> MGERPPPKRLTREAMRNYLKERGDQTVLILHAKVAQKSYGNEKRFFCPPPCVYLMGSGWKKKKEQMERDGCSEQESQPCAFIGIGNSDQEMQQLNLEGKNYCTAKTLYISDSDKRKHFMLSVKMFYGNSDDIGVFLSKRIKVISKPSKKKQSLKNADLCIASGTKVALFNRLRSQTVSTRYLHVEGGNFHASSQQWGAFFIHLLDDDESEGEEFTVRDG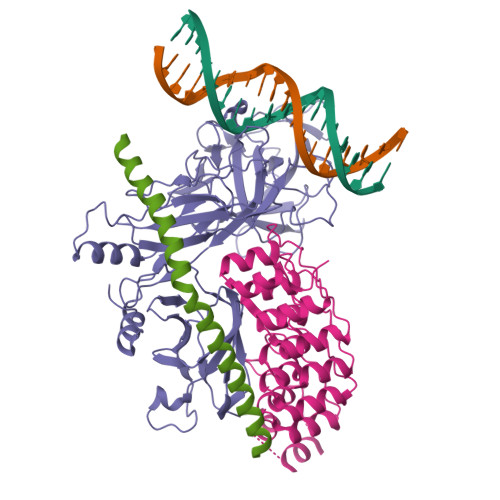YIHYGQTVKLVCSVTGMALPRLIIRKVDKQTALLDADDPVSQLHKCAFYLKDTERMYLCLSQERIIQFQATPCPKEPNKEMINDGASWTIISTDKAEYTFYEGMGPVLAPVTPVPVVESLQLNGGGDVAMLELTGQNFTPNLRVWFGDVEAETMYRCGESMLCVVPDISAFREGWRWVRQPVQVPVTLVRNDGIIYSTSLTFTYTPEPGHHHHHH;> GMDVNVRGPDGFTPLMIASCSGGGLETGNSEEEEDAPAVISDFIYQGASLHNQTDRTGETALHLAARYSRSDAAKRLLEASADANIQDNMGRTPLHAAVSADAQGVFQILIRNRATDLDARMHDGTTPLILAARLAVEGMLEDLINSHADVNAVDDLGKSALHWAAAVNNVDAAVVLLKNGANKDMQNNREETPLFLAAREGSYETAKVLLDHFANRDITDHMDRLPRDIAQERMHHDIVRLLDEYNLVRSPQLHG;> GLPRHSAVMERLRRRIELCRRHHSTCEARYEAVSPERLELERQHTFALHQRCIQAKAKRAGKH>MGSSHHHHHHSSGRENLYFQGDIPQQLVERLQEEKRIEAQKRKERQEAHLYMQVQIVAEDQFCGHQGNDMYDEEKVKYTVFKVLKNSSLAEFVQSLSQTMGFPQDQIRLWPMQARSNGTKRPAMLDNEADGNKTMIELSDNENPWTIFLETVDPELAASGATLPKFDKDHDVMLFLKMYDPKTRSLNYCGHIYTPISCKIRDLLPVMCDRAGFIQDTSLILYEEVKPNLTERIQDYDVSLDKALDELMDGDIIVFQKDDPENDNSELPTAKEYFRDLYHRVDVIFCDKTIPNDPGFVVTLSNRMNYFQVAKTVAQRLNTDPMLLQFFKSQGYRDGPGNP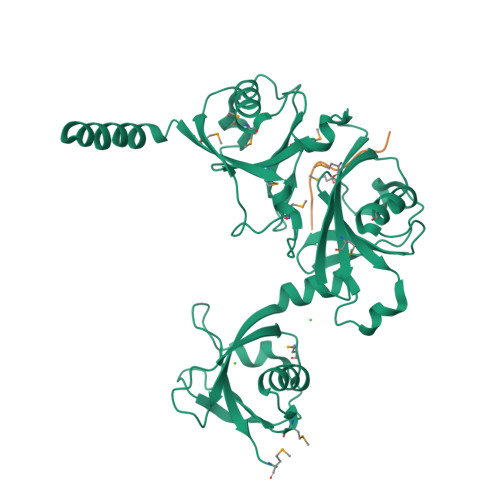LRHNYEGTLRDLLQFFKPRQPKKLYYQQLKMKITDF[2x];>GPRKCARKTRH[2x]> GHMQETQAVEAGEKTVEQFVQALNKGDYNKAAEMTSKKAANKSALSEKEILDKYQNIYGAADVKGLQISNLKVDKKDDSTYSFSYKAKMNTSLGELKDLSYKGTLDRNDGQTTINWQPNLVFPEMEGNDKVSLTTQEAARGNIIDRNGEPLATTGKLKQLGVVPSKLGDGGEKTANIKAIASSFDLTEDAINQAISQSWVQPDYFVPLKIIDGATPELPAGATIQEVDGRYYPLGEAAAQLIGYVGDITAEDIDKNPELSSNGKIGRSGLEMAFDKDLRGTTGGKLSITDADGVEKKVLIEHEVQNGKDIKLTIDA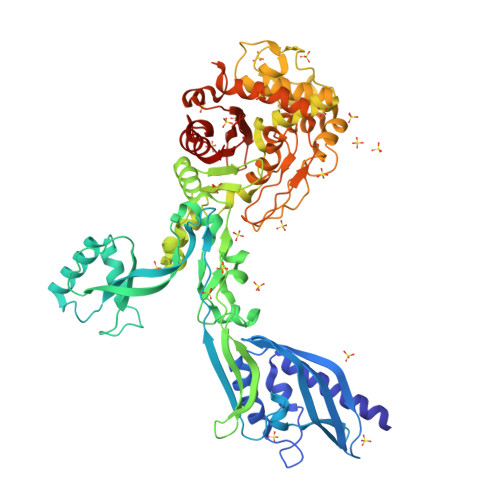KAQKTAFDSLGGKAGSTVATTPKTGDLLALASSPSYDPNKMTNGISQEDYKAYEENPEQPFISRFATGYAPGSTFKMITAAIGLDNGTIDPNEVLTINGLKWQKDSSWGSYQVTRVSSDVSQVDLKTALIYSDNIYTAQETLKMGEKKFRTGLDKFIFGEDLDLPISMNPAQISNEDSFNSDILLADTGYGQGELLINPIQQAAMYSVFANNGTLVYPKLIADKETKDKKNVIGETAVQTIVPDLREVVQDVNGTAHSLSALGIPLAAKTGTAEIKEKQDVKGKENSFLFAFNPDNQGYMMVSMLENKEDDDSATKRASELLQYLNQNYQ>AGHMEAVIEKECSALGGLFQTIISDMKGSYPVWEDFINKAGKLQSQLRTTVVAAAAFLDAFQKVADMATNTRGGTREIGSALTRMCMRHRSIEAKLRQFSSALIDCLINPLQEQMEEWKKVANQLDKDHAKEYKKARQEIKKKSSDTLKLQK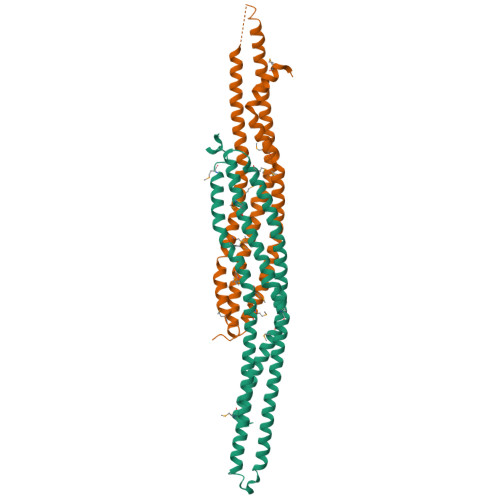KAKKVDAQGRGDIQPQLDSALQDVNDKYLLLEETEKQAVRKALIEERGRFCTFISMLRPVIEEEISMLGEITHLQTISEDLKSLTMDPHKLPSSSEQVILD[2x]>[2x]WGNLGHETVAYIAQSFVASSTESFCQNILGDDSTSYLANVATWADTYKYTDAGEFSKPYHFIDAQDNPPQSCGVDYDRDCGSAGCSISAIQNYTNILLESPNGSEALNALKFVVHIIGDIHQPLHDENLEAGGNGIDVTYDGETTNLHHIWDTNMPEEAAGGYSLSVAKTYADLLTERIKTGTYSSKKDSWTDGIDIKDPVSTSMIWAADANTYVCSTVLDDGLAYINSTDLSGEYYDKSQPVFEELIA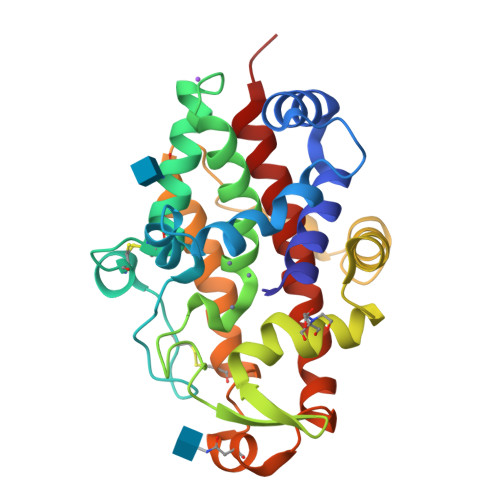KAGYRLAAWLDLIASQPS>MTTVLPPLEDTDGLWAALTEAAASVEKLLATLPEHGARSSAERAEIAAAHDAARALRVRFLDTHADAVYDRLTDHRRVHLRLAELVEAAATAFPGLVPTQQQLAVERSLPQAAKEGHEIDQGIFLRAVLRSPLAGPHLLDAMLRPTPRALELLPEFVRTGEVEMEAVHLERRDGVARLTMCRDDRLNAEDGQQVDDMETAVDLALLDPGVRVGLLRGGVMSHPRYRGKRVFSAGINLKYLSQGGISLVDFLMRRELGYIHKLVRGVLTNDDRPGWWHSPRIEKPWVAAVDGFAIGGGAQLLLVFDRVLASSDAYFSLPCAKEGIIPGAANLRLGRFAGPRVSRQVILEGRR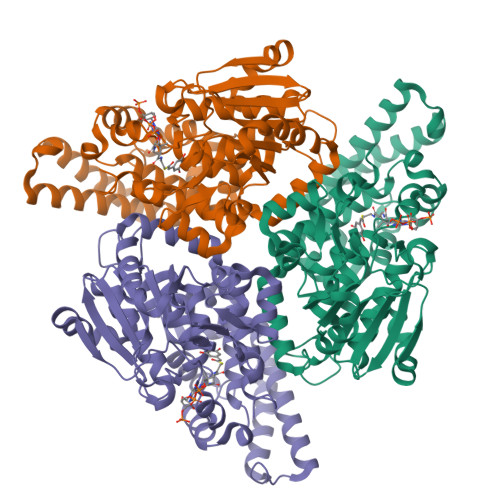IWAKEPEARLLVDEVVEPDELDAAIERSLTRLDGDAVLANRRMLNLADESPDGFRAYMAEFALMQALRLYGHDVIDKVGRFGGRPPA[12x]>[2x]SKIYEDNSLTIGHTPLVRLNRIGNGRILAKVESRNPSFSVACRIGANMIWDAEKRGVLKPGVELVEPTNGNTGIALAYVAAARGYKLTLTMPETMSIERRKLLKALGANLVLTEGAKGMKGAIQKAEEIVASDPQKYLLLQQFSNPANPEIHEKTTGPEIWEDTDGQVDVFISGVGTGGTLT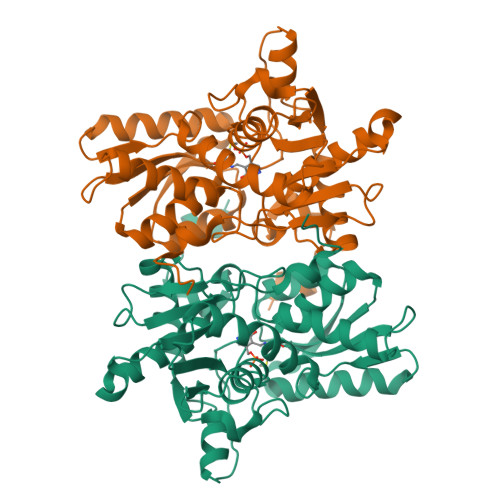GVTRYIKGTKGKTDLITVAVEPTDSPVIAQALAGEEIKPGPHKIQGIGAGFIPGNLDLKLIDKVVGITNEEAISTARRLMEEEGILAGISSGAAVAAALKLQEDESFTNKNIVVILPSSGERYLSTALFADLFTEKELQQ3,7-dihydroxy-2-phenyl-4H-chromen-4-one | C15 H10 O4 | 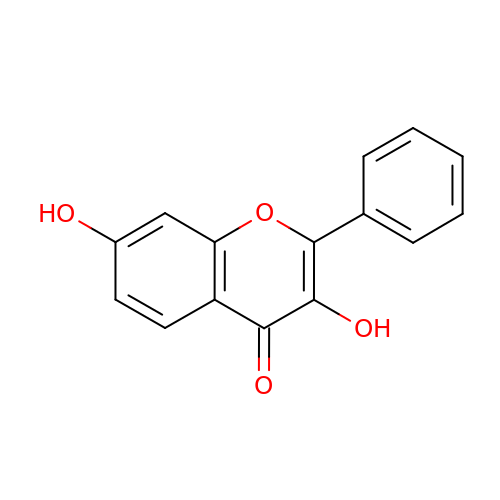UWQJWDYDYIJWKY-UHFFFAOYSA-N>[2x]DVSGTVCLSALPPEATDTLNLIASDGPFPYSQDGVVFQNRESTLPTQSYG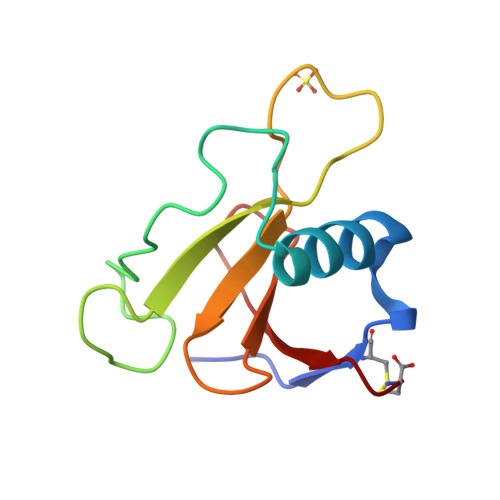YYHEYTVITPGARTRGTRRIITGEATQEDYYTGDHYATFSLIDQTC>AHHHHHHGGAEPIEVITPAKITEPEKVELGKMLFFEPRLSKSGFISCNSCHNLSTGGVDALPTSIGHHWQEGPINSPTVLNADFMLAQFWDGRASNLKEQAAGPIAN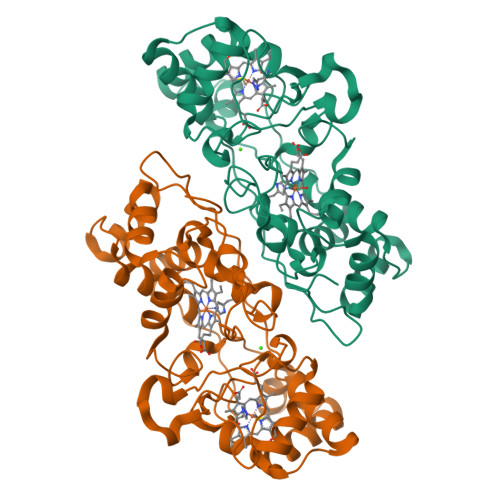PKEMGFTHELATETIASMPAYRARFAKVYGDEKVDIDRLTDAIAAFEKTLVTPNSPFDQYLLGKQDAISGDAKAGYQLFKDKGCVSCHNGPAVGGTMFMKMGLIKPFHTNNPAEGRKGVTGKDADKFVFKVPTLRNIELTYPYFHDGSVWTLEEAVNTMADIQLGQKLTEKETKEMVAFLNSLTGEQPQISLPILPPSNKETPRPVPFATGAK[4x]>GPGSMHAIEVTETGGPGVLRHVDQPQPQPGHGELLIKAEAIGVNFIDTYFRSGQYPRELPFVIGSEVCGTVEAVGPGVTAADTAISVGDRVVSASANGAYAEFCTAPASLTAKVPDDVTSEVAASALLKGLTAHYLLKSVYPVKRGDTVLVHAGAGGVGLILTQWATHLGVRVITTVSTAEKAKLSKDAGADVVLDYPEDAWQFAGRVRELTGGTGVQAVYDGVGATTFDASLASLAVRGTLALFGAASGPVPPVDPQRLNAAGSVYLTRPSLFHFTRTGEEFSWRAAELFDAINSEAITVAVGGRYPLADALR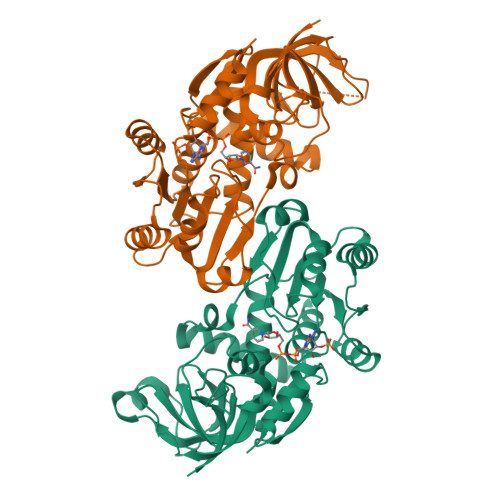AHQDLEARKTVGSVVLLP[4x]> MLEQPYLDLAKKVLDEGHFKPDRTHTGTYSIFGHQMRFDLSKGFPLLTTKKVPFGLIKSELLWFLHGDTNIRFLLQHRNHIWDEWAFEKWVKSDEYHGPDMTDFGHRSQKDPEFAAVYHEEMAKFDDRVLHDDAFAAKYGDLGLVYGSQWRAWHTSKGDTIDQLGDVIEQIKTHPYSRRLIVSAWNPEDVPTMALPPCHTLYQFYVNDGKLSLQLY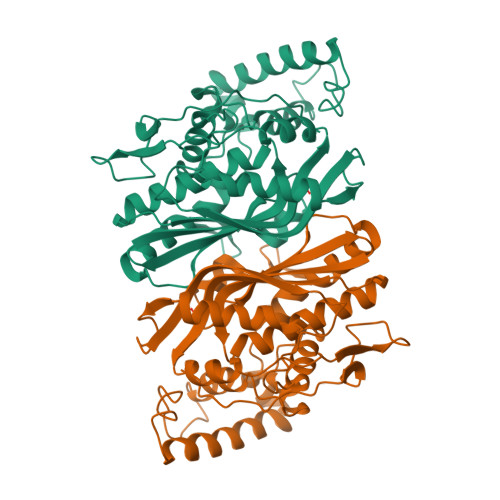QRSADIFLGVPFNIASYALLTHLVAHECGLEVGEFIHTFGDAHLYVNHLDQIKEQLSRTPRPAPTLQLNPDKHDIFDFDMKDIKLLNYDPYPAIKAPVA>GHMARTVNLKGNPVTLVGPELKVGDRAPEAVVVTKDLQEKIVGGAKDVVQVIITVPSLDTPVCETETKKFNEIMAGMEGVDVTVVSMDLPFAQKRFCESFNIQNVTVASDFRYRDMEKYGVLIGEGALKGILARAVFIIDKEGKVAYV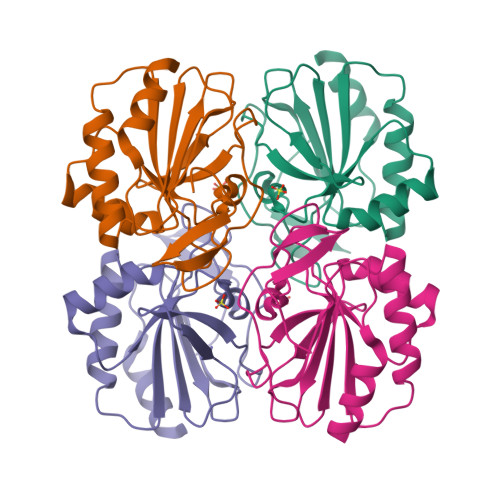QLVPEITEEPNYDEVVNKVKELI[4x]> DPIANAVENAVSALADTTISRVTAASTAASTHSLGTGRVPALQAAETGASSNASDENLIETRCVMNRNGVNEASVEHFYSRAGLVGVVEVKDSGTSLDGYTVWPIDVMGFVQQRRKLELSTYMRFDAEFTFVSNLNDSTTPGMLLQYMYVPPGAPKPDSRKSYQWQTATNPSVFAKLSDPPPQVSVPFMSPATAYQWFYDGYPTFGEHKQATNLQYGQCPNNMMGHFAIRTVSESTTGKNVHVRVYMRIKHVRAWVPRPLRSQAYMVKNYPTYSQTITNTATDRASITTTDYEGGVPANPQRTS;> MGAQVSTEKSGSHETKNVATEGSTINFTNINYYKDSYAASASRQDFAQDPAKFTRPVLDTIREVAAPLQSPSVEACGYSDRVAQLTVGNSTITTQEAANIVLSYGEWPEYCPSTDATAVDKPTRPDVSVNRFYTLSTKSWKTESTGWYWKFPDVLNDTGVFGQNAQFHYLYRSGFCMHVQCNASKFHQGALLVAAIPEFVVAASSPATKPNGQGLYPDFAHTNPGKNGQEFRDPYVLDAGIPLSQALVFP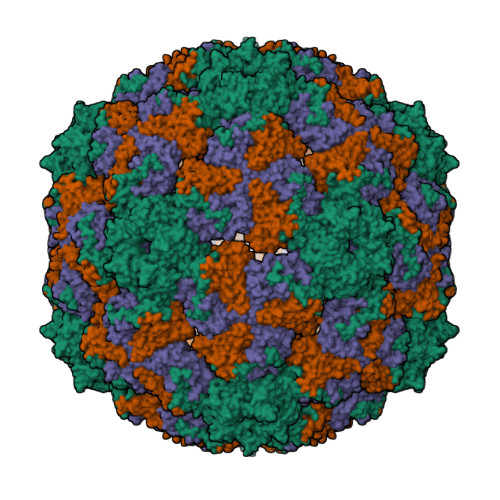HQWINLRTNNCATIIMPYVNALPFDSALNHSNFGLVVIPISPLKYCNGATTEVPITLTIAPLNSEFSGLRQAIKQ;> GFPTELKPGTNQFLTTDDGTSPPILPGFEPTPLIHIPGEFTSLLDLCQIETILEVNNTTSTTGVSRLLIPVRAQNNVDQLCASFQVDPGRNGPWQSTMVGQICRYYTQWSGSLKVTFMFTGSFMATGKMLIAYTPPGSAQPATREAAMLGTHIVWDFGLQSSVTLVIPWISNTHFRAVKTGGVYDYYATGIVTIWYQTNFVVPPDTPTEANIIALGAAQKNFTLKLCKDTDEIQQTAEYQ>[2x]MTSDLIAKLSVNAGEPIGNMRQLHGTSGIPAPAPGTDSVPDILDVWRNAQVTLVRSYDWVSRLDTIDNPTSLFPDWSADPSDPASYNFAATDTWVGQTRSIGANILFTIASEIPANKQPARDLAKYEQVVENIVRHYVCGWGDGFENAVSHWEFGDQPDFGKLHFSGTPDQFYEMYAAAARAVKRVDPALKVGGPCVAFPLNEGP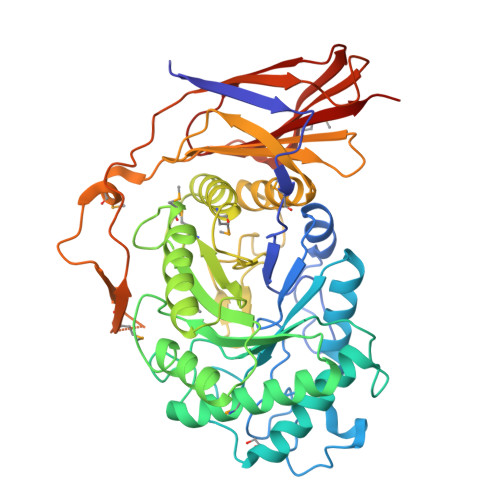FREGFLDYVKQQSVPLDFLSWMWYGDNSRDPMDFRTIAAEVRAIVDKYGFTDTELLLSYWSMTGIPTAKFEDFDNAAFLAAAAIYMQDSEVDKAIFFRADTGADFHYNFTDPAGIFEDDGSQNARTGAFQLVGQTLATTERLAITGGDDNGFAALAGRTADGDTIRILISNYAIPDMYLTARDRDVFEFQVPIGDQKTDMSLNVPPRRVDARSTGYSGYTLEIGHLPWGDGPHRVVRYRADRDHKGEMLDSHEGRGSSVTVQNKLAVSGVELIEITRVSS>MVEINNQRKAFLDMLAWSEGTDNGRQKTRNHGYDVIVGGELFTDYSDHPRKLVTLNPKLKSTGAGRYQLLSRWWDAYRKQLGLKDFSPKSQDAVALQQIKERGALPMIDRGDIRQAIDRCSNIWASLPGAGYG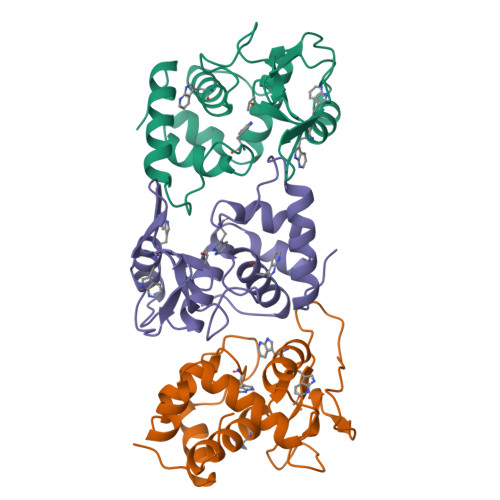QFEHKADSLIAKFKEAGGTVREIDV[3x]(1S,2S)-N-[(6P)-8-amino-6-(4-methylpyridin-3-yl)isoquinolin-3-yl]-2-cyanocyclopropane-1-carboxamide | C20 H17 N5 O | 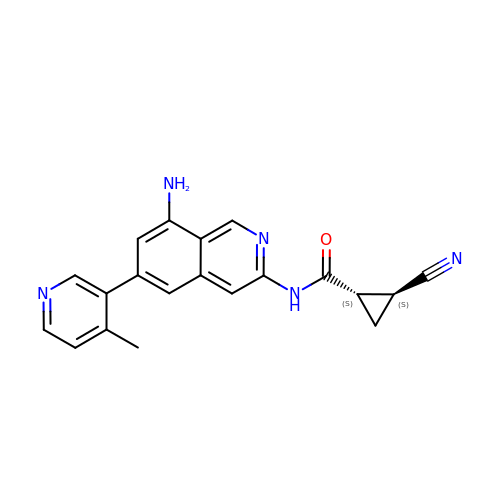DKSAUTCUJKILFS-CABCVRRESA-N>MLDEKSSNTASVVVLCTAPDEATAQDLAAKVLAEKLAACATLIPGATSLYYWEGKLEQEYVVQMILKTTVSHQQ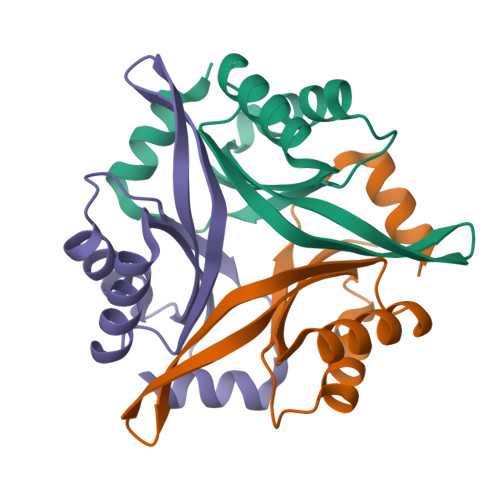ALLECLKSHHPYQTPELLVLPVTHGDTDYLSWLNASLR[3x]> HHHHMVDAAVAEKLEAGFQKLQEATNCKSLLKKHLTREIFDKIKDLKTSFGSTLLDVIQSGVENLDSGFGVYAPDAEAYSVFNDLFEPMICDYHTGFKPGDAHPPRDFGDLETFGNLDPEGAFIVSTRVRCGRSLAGYAFNPCLTEANYKEMEEKVVASLSSLEGELKGTYYPLTGMTKEVQTQLIQDRFLFKEGDRFLQAANACRYWPTGRGIYHNDAKTFLVWCNEEDALRIISMQKGGDLKAVYARLVNAINEIEKRIPFSHHDKYGFLTFCPTNLG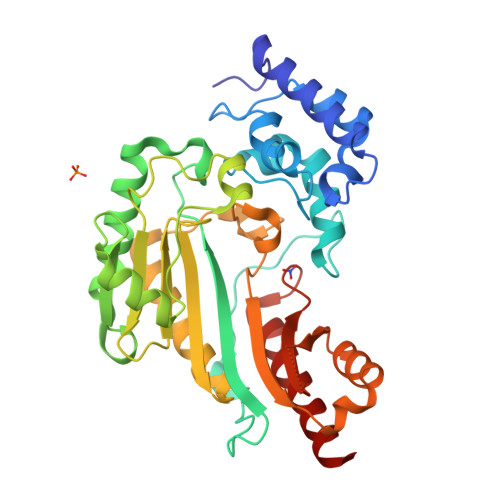TTIRASVHIALPKLAADLAKLEEAAGKFNLQVRGTAGEHTEAEGGVYDISNKRRMGLTEYQAVKEMYDGLQELIRMEKEA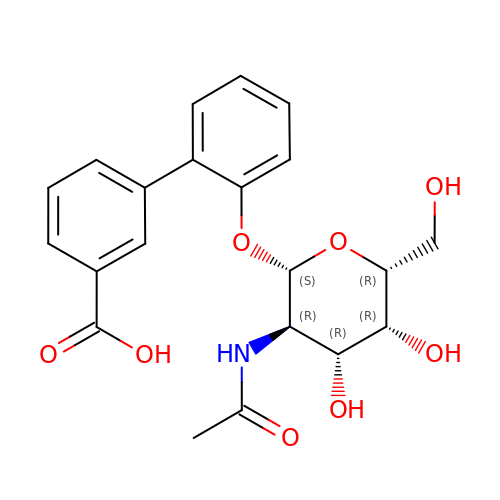ortho-biphenyl-2'-carboxyl N-acetyl-beta-galactosaminoside | C21 H23 N O8 | FLXAKMSHXBTMLT-GQUPQBGVSA-N> HHHHHHSQDPNSSPSSENLYFQSPAPPPVAVVTAPISLSAAIDVQNKLHKTIGVFLPLSTFITRA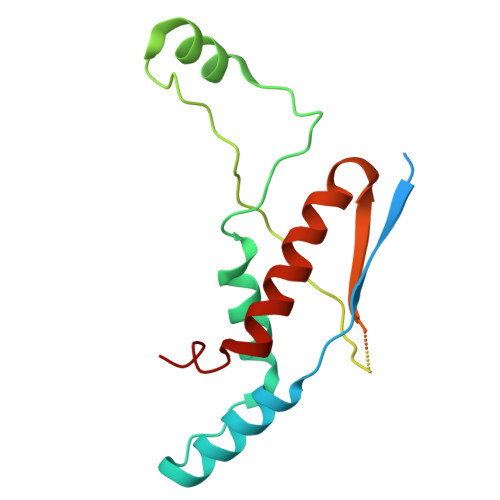TEIANQKLPLPANYQPTADELFNQVLGLDKVTRKESRGSYTPTFGSFVAPQRAARKADIIDILAAPSTRVAASAQSKSAAPGLTTSGPNVFSLQVPKSEEKRAQAFLQKMKLVLEQEPDKLVRA> MIVNVIQKDRLKEQKLQFIRNHQQAFDVEPIYPLPLFEDFVTSIEGDCSLEASCKIESDKLIASRFLLFFEDKTQEWQKYLHQSLTFFGLVENRVGVKINYSLLQQFLGSSFDFSKVTVLSAGIDLRNNLAESSLKMHIRIKDYPEKLDKAFALSDGAA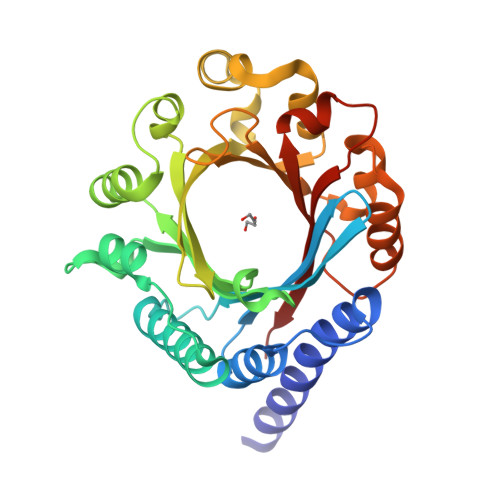DGNYLKDFVNLIGFDFYFNGKSEIEIYAEVQEDDFFKPEINNLVWQHFPKTALQPLKASSLFFTGLSKANNNPVLYYHLKNRQDLTNYFKLNDTAQRVHSFYQHQDILPYMWVGTAQKELEKTRIENIRLYYYKSFKMESN> MTGPIVYVQNADGIFFKLAEGKGTNDAVIHLANQDQGVRVLGAEEFPVQGEVVKIASLMGFIKLKLNRYAIIANTVEETGRFNGHVFYRVLQHSIVSTKFNSRIDSEEAEYIKLLELHLKNSTFYFSYTYDLTNSLQRNEKVGPAASWKTADERFFWNHYLTEDLRNFAHQDPRIDSFIQPVIYGYAKT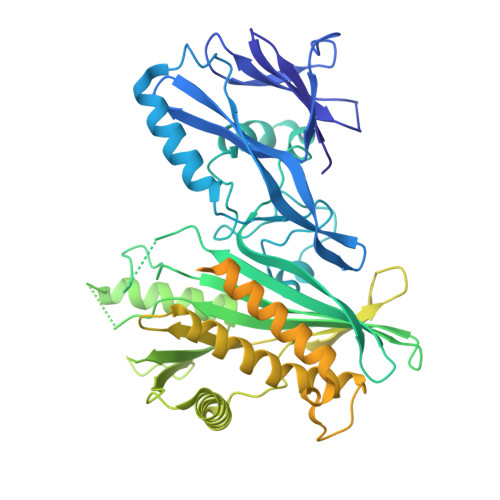VDAVLNATPIVLGLITRRSIFRAGTRYFRRGVDKDGNVGNFNETEQILLAENPESEKIHVFSFLQTRGSVPIYWAEINNLKYKPNLVLGENSLDATKKHFDQQKELYGDNYLVNLVNQKGHELPVKEGYESVVHALNDPKIHYVYFDFHHECRKMQWHRVKLLIDHLEKLGLSNEDFFHKVIDSNGNTVEIVNEQHSVVRTNCMDCLDRTNVVQSVLAQWVLQKEFESADVVATGSTWEDNAPLLTSYQNLWADNADAVSVAYSGTGALKTDFTRTGKRTRLGAFNDFLNSASRYYQNNWTDGPRQDSYDLFLGGFRPHTASIKSPFPDRRPVYIQLIPMIICAALTVLGATIFFPKDRFTSSKNLLYFAGASIVLALSTKFMFKNGIQFVNWPKLVDVGFLVVHQTHDKEQQFKGLKYAQSPKFSKPDPLKRD3-{2-[(4-carbamimidoylphenyl)carbamoyl]-4-ethenyl-5-methoxyphenyl}-6-[(cyclopropylmethyl)carbamoyl]pyridine-2-carboxylic 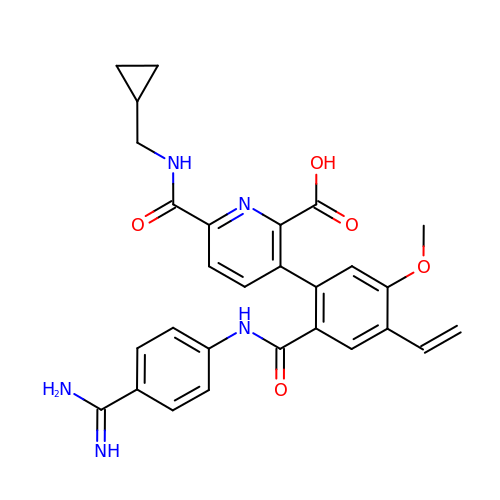acid | C28 H27 N5 O5 | TUWMKPVJGGWGNL-UHFFFAOYSA-N2-(fluorosulfonyl)benzene-1-sulfonic 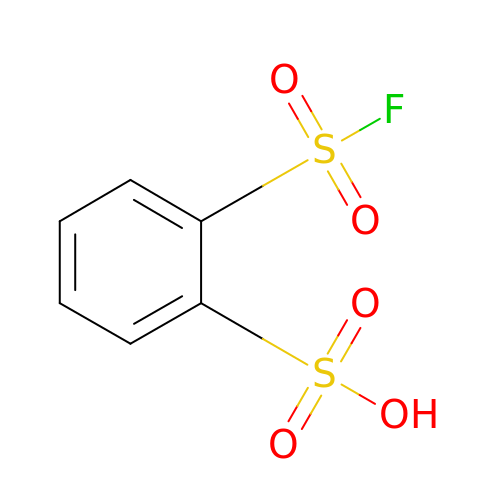acid | C6 H5 F O5 S2 | AFQCDYWSMCQAJJ-UHFFFAOYSA-N> LEEYDKIQKKMEDVMEGKGKLTLRD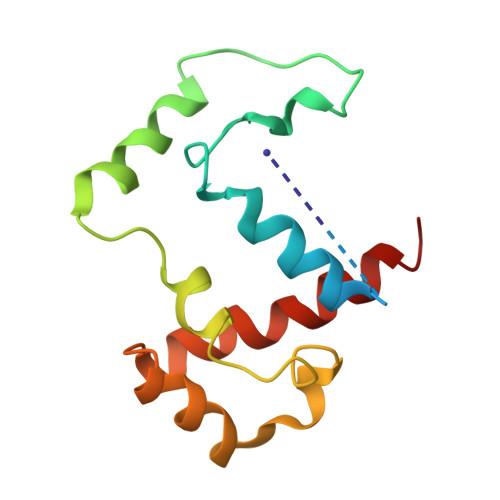VYAQIIALRKMGPLSKVLQHIPGLGIMLPTPSEDQLKIGEEKIRRWLAALNSMTYKELENPNIIDKSRMRRIAEGSGLEVEEVRELLEWYNNMNRLLKMV> KYKK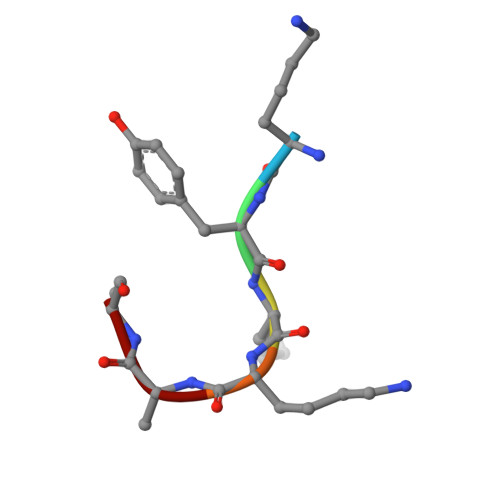AL> SGTTNTVAAYNLTWKSTNFKTILEWEPKPVNQVYTVQISTKSGDWKSKCFYTTDTECDLTDEIVKDVKQTYLARVFSYPAGNVESTGSAGEPLYENSPEFTPYLETNLGQPTIQSFEQVGTKVNVTVEDERTLVRRNNTFLSLRDVFGKDLIYTLYYWKSSS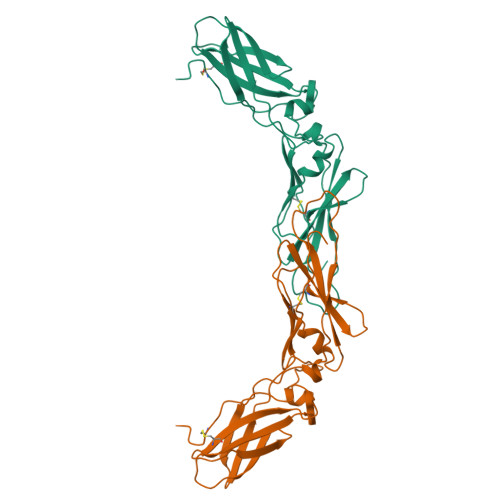SGKKTAKTNTNEFLIDVDKGENYCFSVQAVIPSRTVNRKSTDSPVECMGQEKGEFRE> MAKQIKGIAASDGVAIAKAYLLVEPDLSFDNESVTDTDAEVAKFNGALNKSKVELTKIRNNAEKQLGADKAAIFDAHLLVLEDPELIQPIEDKIKNESVNAAQALTDVSNQFITIFESMDNEYMAERAADIRDVSKRVLAHILGVELPNPSIVDESVVIIGNDLTPSDT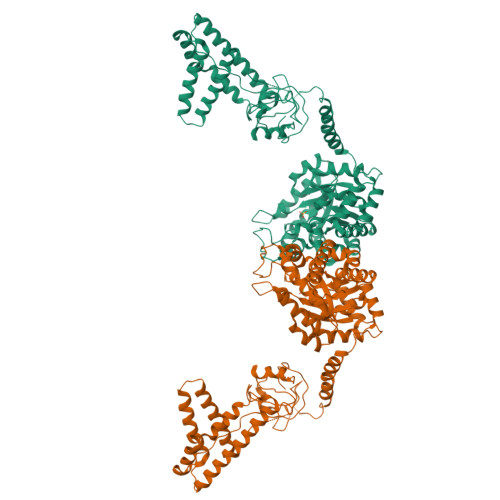AQLNKEYVQGFVTNIGGRTSHSAIMSRSLEIPAVVGTKSITEEVEAGDTIVVDGMTGDVLINPSDEVIAEYQEKRENFFKDKQELQKLRDAESVTADGHHVELAANIGTPNDLPGVIENGAEGIGLYRTEFLYMGRDQMPTEEEQFEAYKAVLEAMKGKRVVVRTLDIGGDKELPYLDLPEEMNPFLGYRAIRLCLDQPEIFRPQLRALLRASVFGKLNIMFPMVATIQEFRDAKALLEEERANLKNEGYEVADDIELGIMVEIPSTAALADIFAKEVDFFSIGTNDLIQYTMAADRMSERVSYLYQPYNPAILRLVKQVIEASHAEGKWTGMCGEMAGDQTAIPLLLGLGLDEFSMSATSILKARRLIRSLNESEMKELSERAVQCATSEEVVDLVEEYTKNA>VMAKKTMGIHHITAIVGHPQENTDFYAGVLGLRLVKQTVNFDDPGTYHLYFGNEGGKPGTIITFFPWAGARQGVIG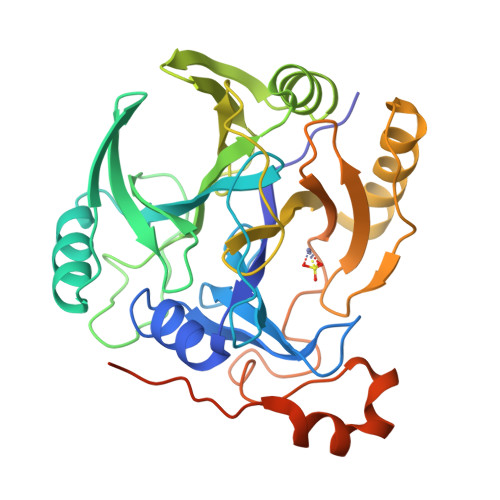DGQVGVTSYVVPKGAMAFWEKRLEKFNVPYTKIERFGEQYVEFDDPHGLHLEIVEREEGEANTWTFGEVTPDVAIKGFGGATLLSEQPDKTADLLENIMGLERVGKEGDFVRYRSAGDIGNVIDLKLTPIGRGQMGAGTVHHIAWRANDDEDQLDWQRYIASHGYGVTPVRDRNYFNAIYFREHGEILFEIATDPPGFAHDETQETMGEKLMLPVQYEPHRTQIEQGLLPFEVRELDAENLYFQSHHHHHHWSHPQFEK[2x]> GKEKLPKMRLPTRSDMICGYACLKGTAAMRNTKRGSWYIEALAQVFSERACDMHVADMLVKVNALIKDREGYAPGTEFHRCKEMSEYCSTLC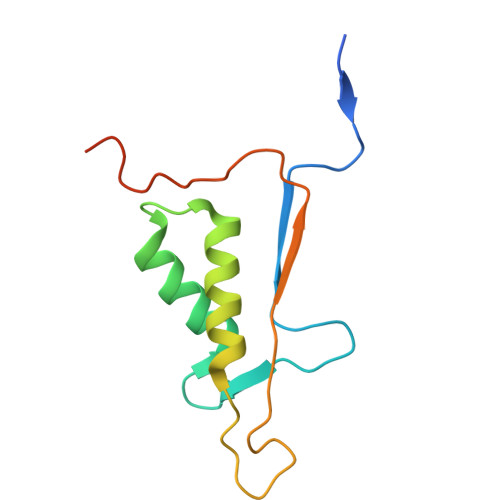RHLYLFPGHPPTLEHHHHHH> GSHMVQLVNFLQSEHPQTIAVVLSYLDPPVAA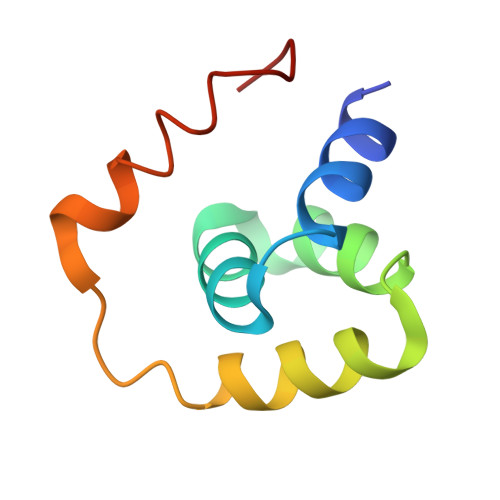QILGALPEELQTEVLKRIALLERTSPEVVKEIERNLEKKISGF>[2x]MDAPLLHIAMFPWFAMGHLTPYLHLSNKLAKRGHKISFIVPKRTQTKLQHLNLHPHLITFVPITVPHIDGLPHDAETTSDVPFSLFTLIATAMDRTEKDIELLLRDLKPQIVFFDFQHWLPNLTRSLGIKSVQYLIVNPITPAYLGNRPKGRDITEADLMQPPPGFPGSAIKLHSHELRFLISTRKLEFGSGVLFLDRLSIGTRLSDAVAFKGCREIEGPYAEYLETVYGKPFLLSGPLLPEPSISTLEEKWVAWLGGFKAGSVIYCAYGSESPLQYNQFLELLLGLELTGFPFLAALKPPAGFETIEEALPEGFRERVEGRGIAYGGWVQQQMILEHPSVGCFITHCGAASITEGLVNTCQLVLLPRLGSDHIMNARLMSTKLKVGVEVEKGEEDGLFTKESVCKAVKIVMDEENEIGREVRANHTKVRNLLLSNNLESSCVDTFCDRLRGLL

In plant biosynthesis, the formation of glycosidic bond is usually catalyzed by uridine diphosphate-dependent glycosyltransferases (UGTs). In this work, we report an efficient phenolic apiosyltransferase GuApiGT from G. uralensis, and dissect mechanisms for its sugar donor selectivity towards UDP-Api through crystal structure analysis, theoretical calculations, and mutagenesis. GuApiGT could efficiently and regio-selectively catalyze 2″-O-apiosylation of flavonoid glycosides, and showed strict sugar donor selectivity towards UDP-Api. This selectivity was highly related with the unique 45-amino acid PSPG box and the key RLGSDH sugar binding motif. Through theoretical calculations and rational design, we altered the sugar donor selectivity of GuApiGT and Sb3GT1.

In order to dissect the mechanisms, we obtained the apo crystal structure of GuApiGT with a resolution of 2.2 Å. Due to the low amino acid sequence identity with reported structures, the structure of GuApiGT was solved by molecular replacement with the help of AlphaFold2 simulation. The crystal contains two highly similar molecules with a root mean square deviation (RMSD) of 1.1 Å, and adopts a canonical GT-B fold consisting of two Rossmann-like β/α/β domains that face each other and are separated by a deep cleft. The N-terminal domain (NTD, residues 1-242 and 436-454) and the C-terminal domain (CTD, residues 243-435) are responsible primarily for sugar acceptor and sugar donor binding, respectively. Based on the structures of GgCGT/UDP-Glc, GgCGT/UDP-Gal, and UGT89C1/UDP-Rha, we simulated the UDP-Api binding pocket of GuApiGT. It is noteworthy that a part of UDP-sugar binding region of GuApiGT is different from that of GgCGT (glucosyltransferase), SbCGTb (arabinosyltransferase), or UGT89C1 (rhamnosyltransferase). Moreover, the plant secondary product glycosyltransferase box (PSPG box) of GuApiGT contains 45 amino acids due to the additional S371 residue. Representative snapshots of GuApiGT/UDP-Api/2 complex model indicate that D372, H373, and I136 could form hydrogen bonds with the apiose OH group. Moreover, R368 could change its initial state, and the side chain could flip into the pocket to form π-π/cation-π interactions and hydrogen bonds with H373, and hydrogen bonds with UDP. We propose that the additional S371 residue could increase flexibility of the loop, thus enables R368 to interact with H373 for the binding of UDP-Api.> EDDDIKQLA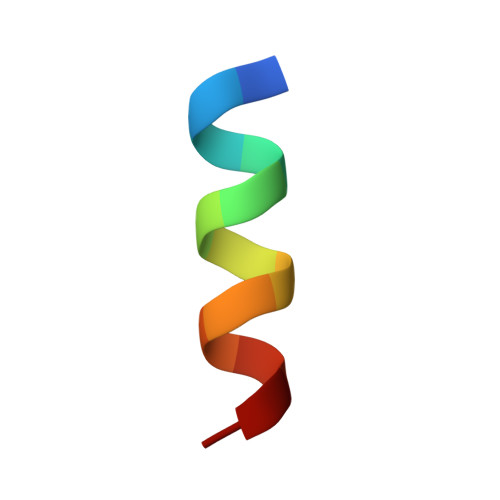AWAT ADENOSINE | C10 H13 N5 O4 | 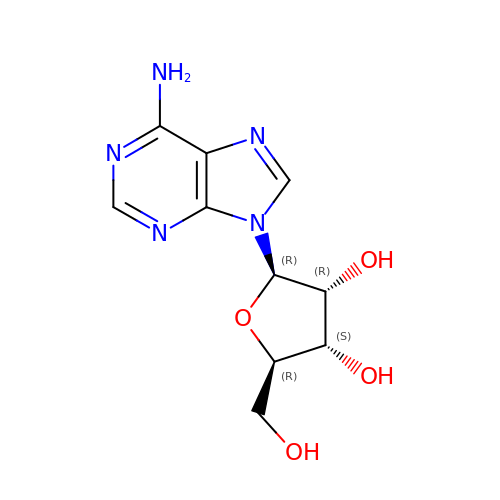OIRDTQYFTABQOQ-KQYNXXCUSA-N>[6x]GSMIRSMTAYARREIKGEWGSATWEMRSVNQRYLETYFRLPEQFRSLEPVVRERIRSRLTRGKVECTLRYEPDVSAQGELILNEKLAKQLVTAANWVKMQSDEGEI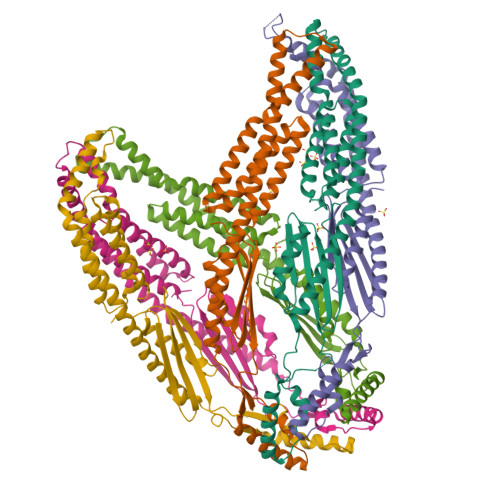NPVDILRWPGVMAAQEQDLDAIAAEILAALDGTLDDFIVARETEGQALKALIEQRLEGVTAEVVKVRSHMPEILQWQRERLVTKLEDAQVQLENNRLEQELVLLAQRIDVAEELDRLEAHVKETYNILKKKEAVGRRLDFMMQEFNRESNTLASKSINAEVTNSAIELKVLIEQMREQIQNIE> VFHKIRNEDLIFNESLGQGTFTKIFKGVRREVGDYGQLHETEVLLKVLDKAHRNYSESFFEAASMMSKLSHKHLVLNYG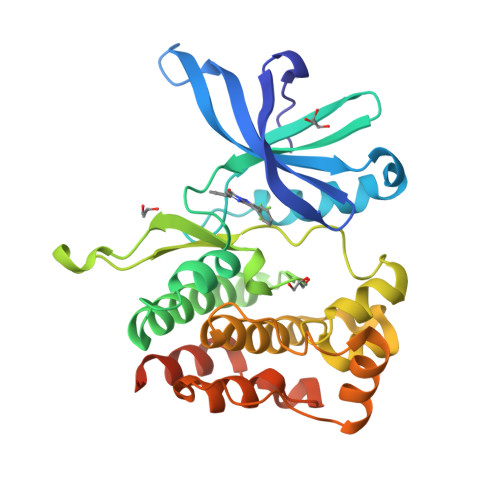VCVCGDENILVQEFVKFGSLDTYLKKNKNCINILWKLEVAKQLAAAMHFLEENTLIHGNVCAKNILLIREEDRKTGNPPFIKLSDPGISITVLPKDILQERIPWVPPECIENPKNLNLATDKWSFGTTLWEICSGGDKPLSALDSERKLQFYEDRHQLPAPKAAELANLINNCMDYEPDHRPSFRAIIRDLNSLFTPDLVPRGSHHHHHH>[6x]SKQDILSLNIPHDINGTERSTQKIQLIVKSKYGLDRIVWDDSALRSQGGQIQHSGSQSAQDYQAILPAYVQGGSNVYKVTARAYDRNGNSSNNVLLTITVLSNGQVVDQVGVTDFTADKTSA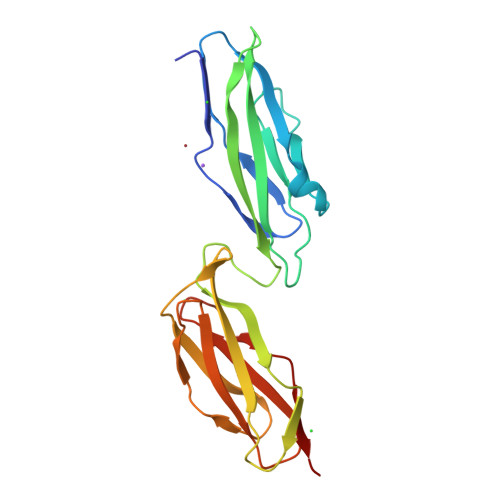KADGTEAITYTATVKKNGVAQANVPVSFNIVSGTAVLSANSANTNGSGKATVTLKSDKPGQVVVSAKTAEMTSALNANAVIFVDQ A periplasmic solute-binding protein (Smon0123) captures unsaturated GAG disaccharides with the 1,3-glycoside bond and delivers substrates to an ABC transporter localized in the cytoplasmic membrane. Smon0123 is composed of two major domains (N- and C-domains), and each domain has two small subdomains. Each domain included a parallel and an antiparallel β-sheet surrounded by many α-helices and formed the α/β sandwich structure. All the crystal structures of Smon0123 so far determined include metal ion in its molecule, suggesting that the metal ion contributes to protein folding.

Crystal structures of ligand-free Smon0123 (N-28/C-5) and ligand (CΔ4S or CΔ6S)-bound Smon0123 (N-18/C-5) were also determined by molecular replacement with CΔ0S-bound Smon0123 (N-18/C-5). Compared with the structure of CΔ0S-bound Smon0123 and that of ligand-free Smon0123, the N- and C-domains of ligand-bound Smon0123 were 47° more closed than those of ligand-free Smon0123. There was no significant difference in the overall structure among Smon0123 proteins in complex with CΔ0S, CΔ4S, and CΔ6S. Unsaturated GAG disaccharides were bound to the cleft of Smon0123 by hydrogen bonds and van der Waals (C-C) contacts. Smon0123 strictly recognized both residues of unsaturated uronate (ΔGlcUA) and amino sugar (GalNAc/GalNAc4S/GalNAc6S). An aromatic residue, Trp284, showed stacking interactions with both ΔGlcUA and GalNAc/GalNAc4S/GalNAc6S. The numbers of hydrogen bonds between Smon0123 and unsaturated chondroitin disaccharides are 9 for CΔ0S (ΔGlcUA, 4; GalNAc, 5), 14 for CΔ4S (ΔGlcUA, 4; GalNAc4S, 10), and 8 for CΔ6S (ΔGlcUA, 4; GalNAc6S, 4). The numbers of C-C contacts between Smon0123 and unsaturated chondroitin disaccharides are 50 for CΔ0S (ΔGlcUA, 27; GalNAc, 23), 48 for CΔ4S (ΔGlcUA, 26; GalNAc4S, 22), and 53 for CΔ6S (ΔGlcUA, 28; GalNAc6S, 25). The sulfate group of each substrate is situated close to the binding site of Smon0123 and directly forms hydrogen bonds with several residues of Smon0123.

>MKKEETTTGPKETTIFAMHLGKALDPNLPVFVKAEKDTNIKLVNVASQNQTDQIQAYNLMLTEGKLPDIVSYELSADLENLGIEGGLIPLEDLINQHAPNLKKFFEENPRYKKDAVAVDGHIYMIPNYYDYFNIKVSQGYFIRQDWLEKLGLKEPRTVDELYTTLKAFREKDPNGNGKKDEVPFFVRANNVRKVLTSLVDLFKASPIWYEENGMVKYGPAQKEFKHAIKELSKWYKEGLIDEEIFTRGLESRDYLLSNNLGGATDDWIASTSSYNRNLADKIPGFNLKLVLPYELNGNAKTRHARTTYLGGWGISKDAKDPVSLIKYFDYWYSVEGRRLWNFGIEGSEYTLVDGKPVFTDKVLKNPDGKTPLAVLREVGAQYRLGAFQDAQYELGWASESAKAGYKYYMDNDVVLDELPILKYTKEKSKEFVSIDTAMRAVVEEKAQQWILGSGDIDKEWDAYIKRLENLGLSKAEQIQNEAF[3x]> MPISPIETVPVKLKPGMDGPKVKQWPLTEEKIKALVEICTEMEKEGKISKIGPENPYNTPVFAIKKKDSTKWRKLVDFRELNKRTQDFWEVQLGIPHPAGLKKKKSVTVLDVGDAYFSVPLDEDFRKYTAFTIPSINNETPGIRYQYNVLPQGWKGSPAIFQSSMTKILEPFRKQNPDIVIYQYMDDLYVGSDLEIGQHRTKIEELRQHLLRWGLTTPDKKHQKEPPFLWMGYELHPDKWTVQPIVLPEKDSWTVNDICKLVGKLNWASQIYPGIKVRQLSKLLRGTKALTEVIPLTEEAELELAENREILKEPVHGVYYDPSKDLIAEIQKQGQGQWTYQIYQEPFKNLKTGKYARMRGAHTNDVKQLTEAVQKITTESIVIWGKTPKFKLPIQKETWETWWTEYWQATWIPEWEFVNTPPLVKLWYQLEKEP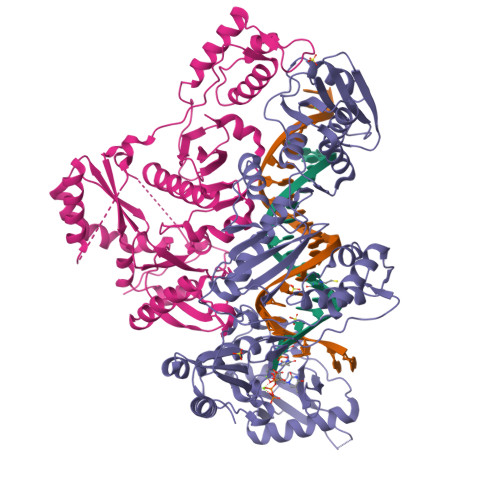IVGAETFYVDGAANRETKLGKAGYVTNRGRQKVVTLTDTTNQKTELQAIYLALQDSGLEVNIVTDSQYALGIIQAQPDQSESELVNQIIEQLIKKEKVYLAWVPAHKGIGGNEQVDKLVSAGIRKVL;> MGSSHHHHHHSSPISPIETVPVKLKPGMDGPKVKQWPLTEEKIKALVEICTEMEKEGKISKIGPENPYNTPVFAIKKKDSTKWRKLVDFRELNKRTQDFWEVQLGIPHPAGLKKKKSVTVLDVGDAYFSVPLDEDFRKYTAFTIPSINNETPGIRYQYNVLPQGWKGSPAIFQSSMTKILEPFRKQNPDIVIYQYMDDLYVGSDLEIGQHRTKIEELRQHLLRWGLTTPDKKHQKEPPFLWMGYELHPDKWTVQPIVLPEKDSWTVNDIQKLVGKLNWASQIYPGIKVRQLSKLLRGTKALTEVIPLTEEAELELAENREILKEPVHGVYYDPSKDLIAEIQKQGQGQWTYQIYQEPFKNLKTGKYARMRGAHTNDVKQLTEAVQKITTESIVIWGKTPKFKLPIQKETWETWWTEYWQATWIPEWEFVNTPPLVKLWYQLEKEPIVGAETF> AIGPVADLTISNGAVSPDGFSRQAILVNDVFPSPLITGNKGDRFQLNVIDNMTNHTMLKSTSIHWHGFFQHGTNWADGPAFVNQCPISTGHAFLYDFQVPDQAGTFWYHSHLSTQYCDGLRGPIVVYDPQDPHKSLYDVDDDSTVITLADWYHLAAKVGSPVPTADATLINGLGRSIDTLNADLAVITVTKGKRYRFRLVSLSCDPNHVFSIDGHSLTVIEADSVNLKPQTVDSIQIFAAQRYSFVLNADQDVGNYWIRALPNSGTRNFDGGV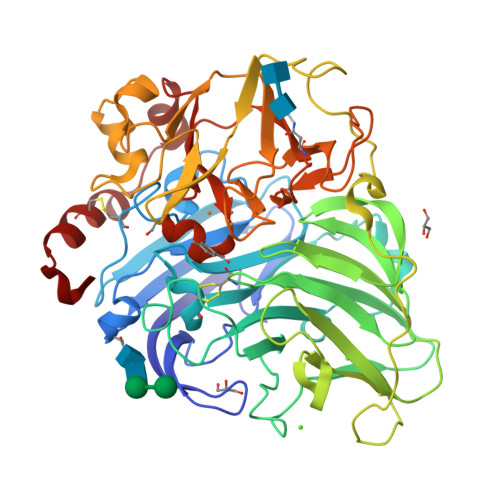NSAILRYDGAAPVEPTTSQTPSTNPLVESALTTLEGTAAPGSPAPGGVDLALNMAFGFAGGKFTINGASFTPPTVPVLLQILSGAQSAQDLLPSGSVYSLPANADIEISLPATAAAPGFPHPFHLHGHTFAVVRSAGSSTYNYENPVYRDVVSTGSPGDNVTIRFRTDNPGPWFLHCHIDFHLEAGFAVVMAEDIPEVAATNPVPQAWSDLCPTYDALSPDDQ>QGYDVEFDPPLESKYECPICLMALREAVQTPCGHRFCKACIIKSIRDAGHKCPVDNEILLENQLFPDNFAKREILSLMVKCPNEGCLHKMELRHLEDHQAHCEFALMDCPQCQRPFQKFH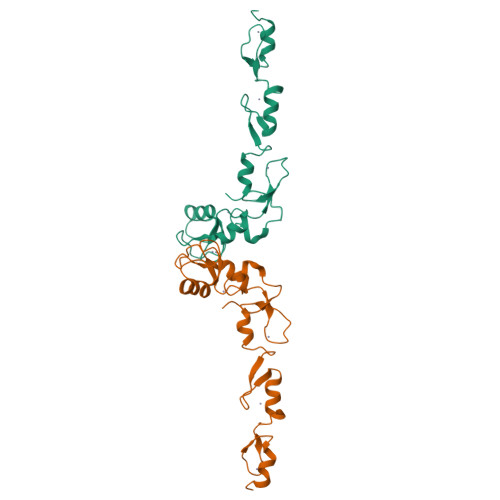INIHILKDCPRRQVSCDNCAASMAFEDKEIHDQNCPL[2x]> LRYDSTAERLY;> ASPISTIQPKANFDAQQFAGTWLLVAVGSAARFLQEQGHRAEATTLHVAPQGTAMAVSTFRKLDGICWQVRQLYGDTGVLGRFLLQARGARGAVHVVVAETDYQSFAVLYLERAGQLSVKLYARSLPVSDSVLSGFEQRVQEAHLTEDQIFYFPKYGFCE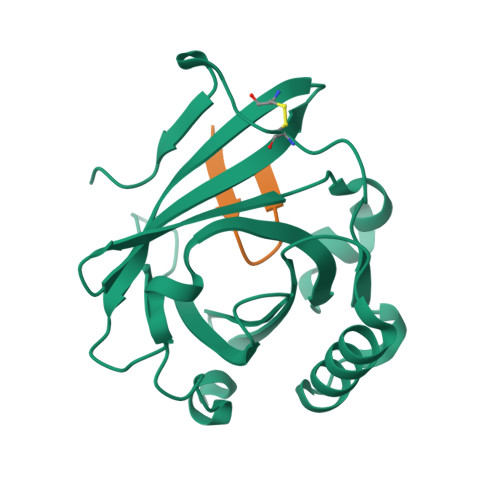AADQFHVLDEVRR>[4x]MGQEPRTLPPSPNWYCARCSDAVPGGLFGFAARTSVFLVRVGPGAGESPGTPPFRVIGELVGHTERVSGFTFSHHPGQYNLCATSSDDGTVKIWDVETKTVVTEHALHQHTISTLHWSPRVKDLIVSGDEKGVVFCYWFNRNDSQHLFIEPRTIFCLTCSPHHEDLVAIGYKDGIVVIIDISKKGEVIHRLRGHDDEIHSIAWCPLPGEDCLSINQEETSEEAEITNGNAVAQAPVTKGCYLATGSKDQTIRIWSCSRGRGVMILKLPFLKRRGGGIDPTVKERLWLTLHWPSNQPTQLVSSCFGGELLQWDLTQSWRRKYTLFSASSEGQNHSRIVFNLCPLQTEDDKQLLLSTSMDRDVKCWDIATLECSWTLPSLGGFAYSLAFSSVDIGSLAIGVGDGMIRVWNTLSIKNNYDVKNFWQGVKSKVTALCWHPTKEGCLAFG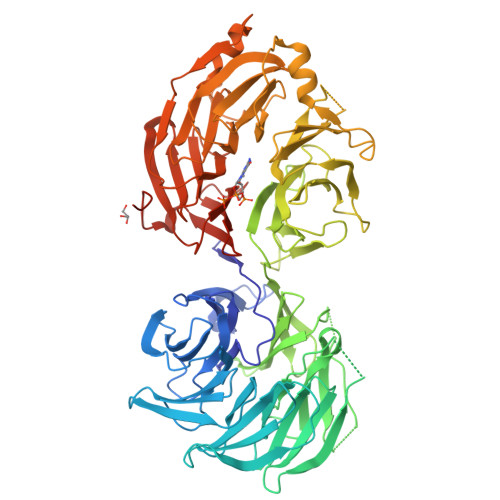TDDGKVGLYDTYSNKPPQISSTYHKKTVYTLAWGPPVPPMSLGGEGDRPSLALYSCGGEGIVLQHNPWKLSGEAFDINKLIRDTNSIKYKLPVHTEISWKADGKIMALGNEDGSIEIFQIPNLKLICTIQQHHKLVNTISWHHEHGSQPELSYLMASGSNNAVIYVHNLKTVIESSPESPVTITEPYRTLSGHTAKITSVAWSPHHDGRLVSASYDGTAQVWDALREEPLCNFRGHRGRLLCVAWSPLDPDCIYSGADDFCVHKWLTSMQDHSRPPQGKKSIELEKKRLSQPKAK>[2x]MIEKMELGEFYKELRLARKLKQTDVACEGLTASQLSKFELGQSMLSADKLILAIQGINVTFDEFGHKLNNYQESPHMRIGRKVVNRFAHQDIAALEQLLEE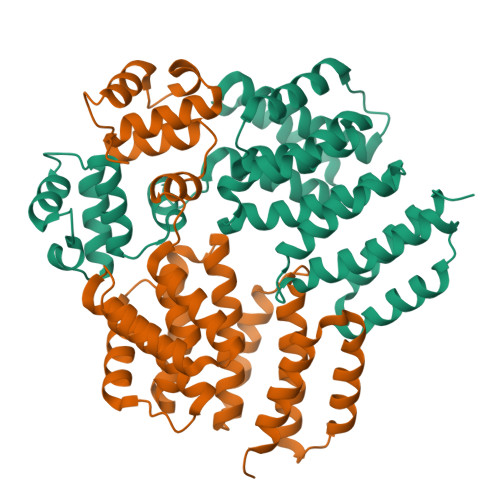VDQEQMAQTYRRLNAIVIKDAIHSLNKSYPLAEEDSEFLTTYLYAIESWTWFELYLFCNTMPFLSNQDLIFLSTSLLEKSKEFKELVHNRLYMKQGLLNILSELMERKLFSYIPIFEAELERMLRPYDVFEKVSWQFLKKMSVFLQTKGSNQKEIERFIQSLQVLENPQLTSLFELRFQQYKELID>MNELKLSKRLQTVAEYIPNGAVMADIGSDHAYLPSYAVLNHKASGAIAGEITDGPFLSAKRQVEKSGLNSHISVRQGDGLEVIKKGEADAITIAGMGGALIAHILEAGKDKLTGKERLILQPNIHAVHIREWLYKERYALIDEVILEEDGKSYEVLVAEAGDRDAAYDGISLSAGMLVGPFLAKEKNAVFLKK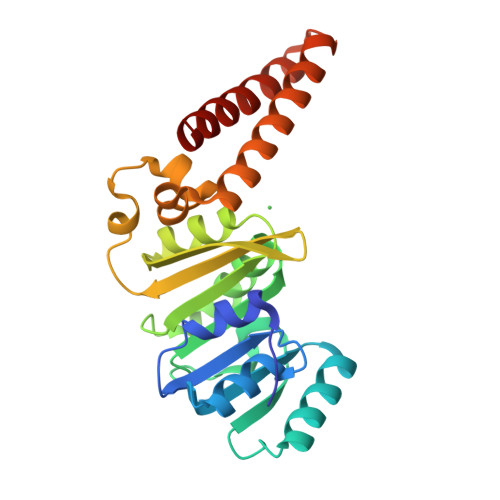WTQELQHTQSIYEQISQAADTEQNKQKLKELADRMELLKEVIDHG[4x]(R)-2-((R)-((R)-2-amino-2-phenylacetamido)(carboxy)methyl)-5-chloro-3,6-dihydro-2H-1,3-thiazine-4-carboxylic 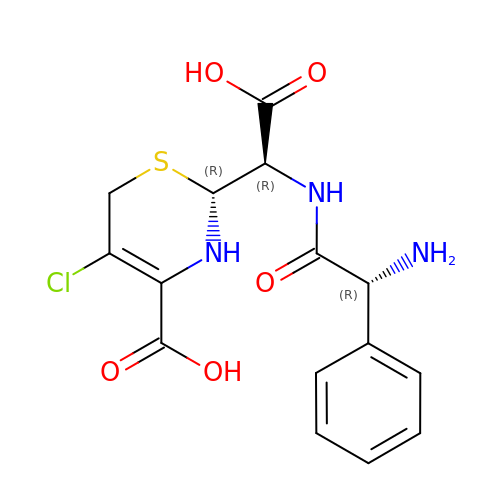acid | C15 H16 Cl N3 O5 S | BPKRUZRKWSLICC-SUZMYJTESA-N> APLTITNRCHFTVWPAVALVLAQGGGGTELHPGASWSLDTPVIGSQYIWGRTGCSFDRAGKGRCQTGDCGGSSLTCGGNPAVPTTMAEVSVL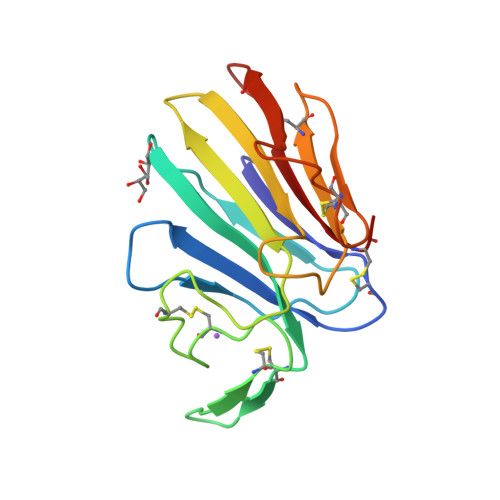QGNYTYGVTSTLKGFNVPMNLKCSSGDALPCRKAGCDVVQPYAKSCSAAGSRLQIVFCP> DDEINAQSVWSEEISSNYPLCIKNLMEGLKKNHHLRYYGRQQLSLFLKGIGLSADEALKFWSEAFTRNGNMTMEKFNKEFRYSFRHNYGLEGNRINYKPWDCHTILSKPRPGRGDYHGCPFRDWSHERLSAELRSMKLTQAQIISVLDSCQKGEYT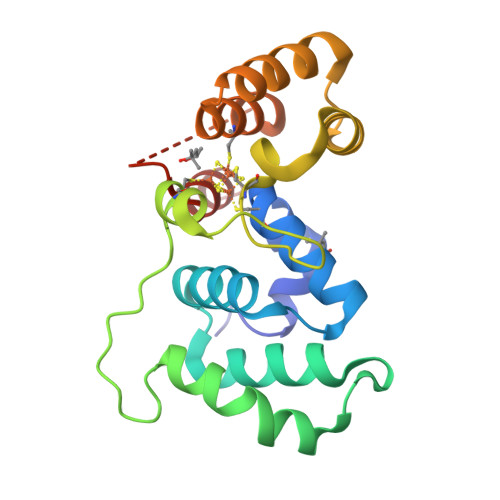IACTKVFEMTHNSASADLEIGEQTHIAHPNLYFERSRQLQK In the bloodstream an unusually tight interaction between the bacteria and the brain microvasculature endothelial cells is established, leading to cortical plaque formation that results in opening of the blood brain barrier and bacterial invasion of the brain. This interaction is mediated by Type IV pili (T4P), long thin polymers of pilin proteins that interact with two endothelial cell receptors, CD147 and the β2 adrenergic receptor (β2AR). The interaction with CD147 is responsible for bacterial adhesion and the interaction with the β2AR induces signalling in endothelial cells. N. meningitidis PilE (Nm PilE) is 78% identical to Ng PilE and 100% identical in α1. Here we report the 1.44 Å X-ray crystal structure of Nm PilE and a cryoEM reconstruction of the Nm pilus at higher resolution, ∼6 Å, than any T4P structure reported previously.

Nm ΔN-PilE is a globular protein with an N-terminal α-helix corresponding to α1C, the C-terminal half of α1, embedded in a four-stranded antiparallel β-sheet (β1 to β4, residues 77–121). Between α1C and the β-sheet is the αβ-loop (residues 54–76), an extended segment with a single-turn α-helix and a 310 helix that forms one edge of the globular domain. Two residues in the αβ-loop, Ser63 and Ser69, are post-translationally modified in the native PilE3940. On the opposite side of the β-sheet, the polypeptide chain exits β4 and forms a β-hairpin (β5–β6) that lies atop the β-sheet, followed by an irregular segment that protrudes from the globular domain surface then wraps under it, ending in an extended C terminus at the edge opposite the αβ-loop. Conserved disulfide-bonded cysteines at the end of β4 (Cys120) and close to the C terminus (Cys154) define the boundaries of the D-region containing the β-hairpin. The most protruding segment of the D-region, the β-hairpin loop and β6 plus the beginning of the loop that follows β6, is highly variable in sequence among N. meningitidis Type IV pilins and is referred to as the hypervariable region (residues ∼127 to 146). The β-hairpin loop hooks over the top of the β-sheet and across the β1–β2 loop; Ala129 at its apex forms a main chain hydrogen bond with Trp57 at the beginning of the αβ-loop. Not surprisingly, the Nm PilE structure is highly similar to Ng PilE, superimposing with a root mean square deviation of 3.1 Å for all main chain atoms. The only notable main chain deviations are in the position of the β3–β4 loop, which bends away from the β-strand in Nm PilE to a greater degree than it does in Ng PilE, and in the β-hairpin, which is more twisted in Nm PilE and has a two-residue insertion in its loop that allows it to contact the αβ-loop. Since the N-terminal 54 residues are identical in both proteins the missing 29 N-terminal residues in Nm ΔN-PilE monomer are also expected to be α-helical, forming a continuous α-helix with α1C, as seen in the full-length Ng PilE structure.

> GSHMARAQVSEAILLAEGQKSAVTEYYLNHGEWPGDNSSAGVATSADIKGKYVQSVTVANGVITAQMASSNVNNEIKSKKLSLWAKRQNGSVKWFCGQPVTRTTATATDVAAANGKTDDKINTKHLPSTCRDDSSAS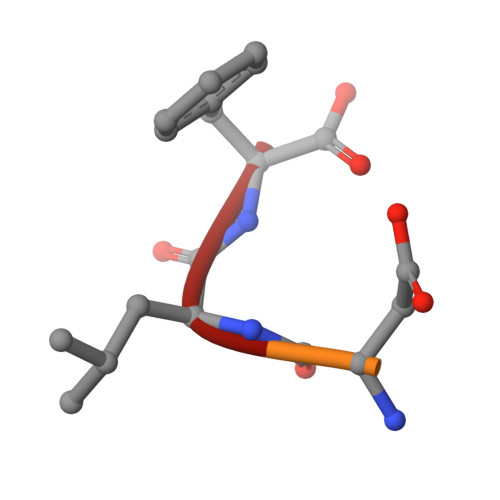> ALDLF>[3x]MRCIGISNRDFVEGVSGGSWVDIVLEHGSCVTTMAKNKPTLDFELIKTEAKQPATLRKYCIEAKLTNTTTESRCPTQGEPSLNEEQDKRFVCKHSMVDRGWGNGCGLFGKGGIVTCAMFRCKKNMEGKVVQPENLEYTVVITPHSGEEHAVGNDTGKHGKEVKITPQSSITEAELTGYGTVTMECSPRTGLDFNEMVLLQMENKAWLVHRQWFLDLPLPWLPGADTQGSNWIQK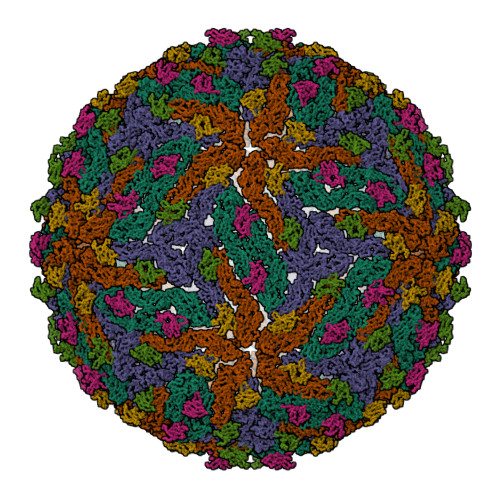ETLVTFKNPHAKKQDVVVLGSQEGAMHTALTGATEIQMSSGNLLFTGHLKCRLRMDKLQLKGMSYSMCTGKFKVVKEIAETQHGTIVIRVQYEGDGSPCKIPFEIMDLEKRHVLGRLITVNPIVTEKDSPVNIEAEPPFGDSYIIIGVEPGQLKLDWFKKG;>FHLTTRNGEPHMIVSRQEKGKSLLFKTEDGVNMCTLMAMDLGELCEDTLTYKCPLLRQNEPEDIDCWCNSTSTWVTYGTCT[3x]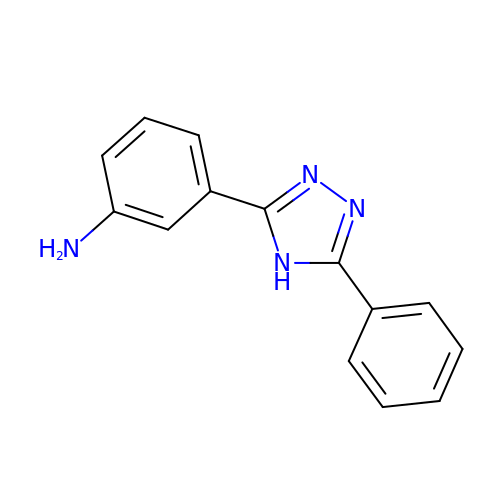3-(5-phenyl-4H-1,2,4-triazol-3-yl)aniline | C14 H12 N4 | KANPBCGVSTVENC-UHFFFAOYSA-N Cytochrome P450 enzymes (CYPs) are heme-containing enzymes that catalyze hydroxylation with a variety of biological molecules. Here, we report the newly identified CYP101D5 from Sphingomonas echinoides. CYP101D5 catalyzes the hydroxylation of β-ionone and flavonoids, including naringenin and apigenin, and causes the dehydrogenation of α-ionone. A structural investigation and comparison with other CYP101 families indicated that spatial constraints at the substrate-recognition site originate from the B/C loop.

For further investigation, the three-dimensional structure of CYP101D5 was determined at a resolution of 3.2 Å using X-ray crystallography. The final model of CYP101D5 contained two molecules in an asymmetric unit, and the two chains were similar to each other, as indicated by 0.620 of Cα RMSD. The overall structure of CYP101D5 showed a typical CYP family fold with 13 α-helices (αA–αL, including αK՛), 8 β-strands (β1–β8), and connecting loops. The heme molecule was located in the central region between the two domains and residues Tyr72 from αB; His105, Arg109, Val112, and Leu116 from αC; Ala251 and The255 from αI; Val298 and Ala300 from the αK–β4 loop; Arg302 from β4; and Thr352, Phe353, His358, Ala361, and Gly362 from the αK’–αL loop, which are mainly involved in the interaction with the heme molecule by a combination of hydrophobic and hydrogen bonding and salt bridges. The active site of CYP101D5 was located at the bottom of the inside of the funnel-like cavity composed of five loops, including the F/G and B/C loops on top of the heme molecule. The analysis indicated that CYP101D5 has two possible pathways. Given that the turn regions of the F/G and B/C loops showed open conformations in the absence of substrates or products, while closed conformations were presented upon a substrate or the product binding of CYPs, such as the CYP105 and CYP101 families, pathway 1 is most likely the substrate access channel for CYP101D5 and changes its conformation during enzymatic catalysis. However, in the structure of CYP101D5, the corresponding loop remained toward the solvent area, and Tyr93 also protruded outwards. We speculated that small amino acids, such as Ala88 and Ala94, are the points that disturb the formation of the helix and cause different conformations. The bent loop of the B/C loop mentioned earlier generates additional space for the substrate in CYP101D5. This conformation of the loop with the outward-pointing tyrosine increases the volume of the active site and enables the hydroxylation of larger substrates.

>MSAAEEIHTPRPAHVPADRVVELDMYNPQGIEKGYLEAWTSLQTADLPSMVWTPLNGGHWIATRGELIQDIYCDPDHFSSHVIFIPKAAGEKYAMVPSKMDPPEHRPYREVVDKGLNLRAIREREPAVRAHAIALIEAFADKGHCDFVEEFSGEFPIRVFMMMADLPMEDSPKLRAFAAGMTRPEGNTPTEMADALDRANRSFFDYVSPIIDARMGGDGTDILTLSINSQVNGAPMEREKLLGMVSLLLLAGLDTVTNFLNMTMDYLGRHPDKVRELTENPTEIRRGVEELFRRFPLVAAARMVAHDVERDGVELKQGEMVLLPTALHGLDPRVNADPWEVDFQRKRPAHSTFGNGPHRCAGLHLARLETTVMLEEWLKRIPTFRVVPGTGPTYHSGVVASVDGVRLEW[2x]> MSLEDYILKVEELNYNYSDGTHALKGINMNIKRGEVTAILGGNGVGKSTLFQNFNGILKPSSGRILFDNKPIDYSRKGIMKLRESIGIVFQDPDNQLFSASVYQDVSFGAVNMKLPEDEIRKRVDNALKRTGIEHLKDKPTHCLSFGQKKRVAIAGVLVMEPKVLILDEPTAGLDPMGVSEIMKLLVEMQKELGITIIIATHDIDIVPLYCDNVFVMKEGRVILQGNPKEV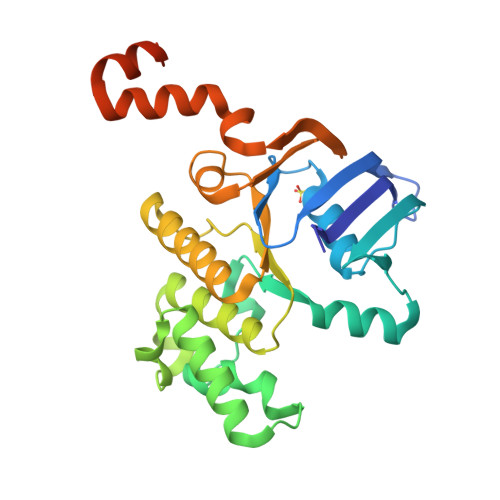FAEKEVIRKVNLRLPRIGHLMEILKEKDGFVFDELDEGHHHHHH>MQIFRDVSKLLVERVDPKILNLFRLLGKFGDEVNMPVYVVGGFVRDLLLGIKNLDIDIVVEGNALEFAEYAKRFLPGKLVKHDKFMTASLFLKGGLRIDIATARLEYYESPAKLPDVEMSTIKKDLYRRDFTINAMAIKLNPKDFGLLIDFFGGYRDLKEGVIRVLHTLSFVDDPTRILRAIRFEQRFDFRIEETTERLLKQAVEEGYLERTTGPRLRQELEKILEEKNPLKSIRRMAQFDVIKHLFPKTYYTPSMDEKMENLFRNIPWVEENFGEVDRFYAVLHVFLEFYDDESWKEVRDRYSLRRNLINEIRHVEKSAPALLEMLSERVPASFVYPLVKGVSNETICHFLAYLSGEKEGLFKSYLLKIKNTKLEKINGEYLIRKGITSGKIIGEVLEKILMKKLDGDTRDE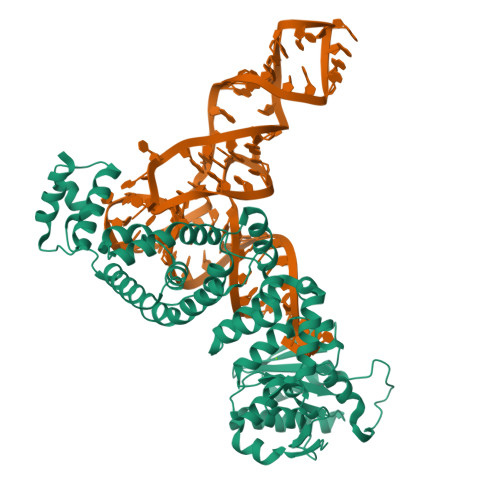EEILEEVLASLETEGKLAAALEHHHHHH[2x]> GYEEREGGFRKETVERLLRLHFRDGRTRVNGDALLLMAELLK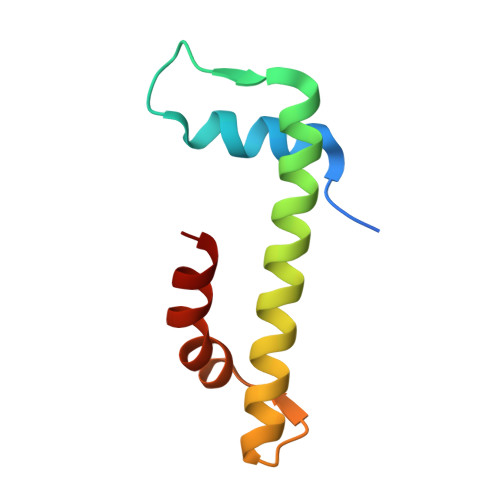VFVREAAARAARQAQAEDLEKVDIEHVEKVLPQLLLDFV> MKHHHHHHMSLDAFEILTTSGVVLWSRTYAPVNPSVVNDFITDVF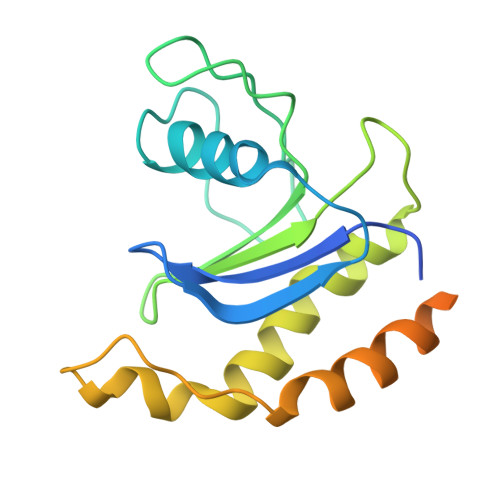IEEKSAVAGSKNGGSAASNPPYKHDQHSLRWTFVKELGIIFVAVYRSLLHLPWVDKLVDNIRAIFVSLYSEQFKRPNTTIIECINFDKYFDQQLQELEQTGSRVDARVPKIEAHSADEEEQPFVPSPAGKSEQKAP>[2x]MKTREIYAEMRCIPPVVLRADGRNFKNTLSGLGFEKPYDKTFARAMADTAELF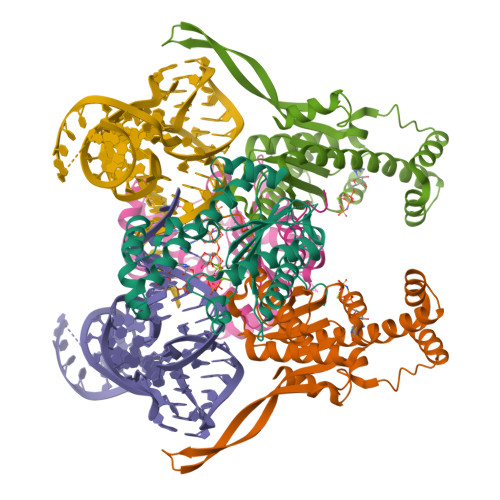IKKSGLSPLFAYTFSDEISFLFTDLPFDGRVEKIDSVVASFLGSALTIKLRLEEPIAFDSRLVALQKEEIPEYFHRRQLEAWRNFVASWGYYALRNEGMGRNEAAKYLKRKKESEIHEMLFERGINLATLPSWQRRGVIISKEAREIQGFNPVSGKEEKSLRRKITQNWEIPKFKSEKGIPFLEKLINRNLEHHHHHH>[3x]MAAIPALDPEAEPSMDVILVGSSELSSSVSPGTGRDLIAYEVKANQRNIEDICICCGSLQVHTQHPLFEGGICAPCKDKFLDALFLYDDDGYQSYCSICCSGETLLICGNPDCTRCYCFECVDSLVGPGTSGKVHAMSNWVCYLCLPSSRSGLLQRRRKWRSQLKAFYDRESENPLEMFETVPVWRRQPVRVLSLFEDIKKELTSLGFLESGSDPGQLKHVVDVTDTVRKDVEEWGPFDLVYGA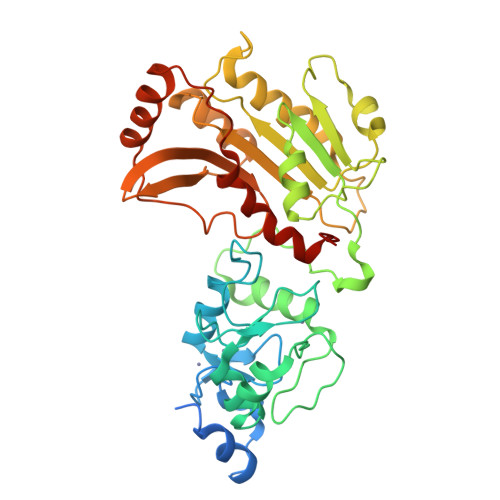TPPLGHTCDRPPSWYLFQFHRLLQYARPKPGSPGPFFWMFVDNLVLNKEDLDVASRFLEMEPVTIPDVHGGSLQNAVRVWSNIPAIRSRHWALVSEEELSLLAQNKQSSKLAAKWPTKLVKNCFLPLREYFKYFSTELTSSL>[2x]VFPCSVYVPDEWEVSREKITLLRELGQGSFGMVYEGNARDIIKGEAETRVAVKTVNESASLRERIEFLNEASVMKGFTCH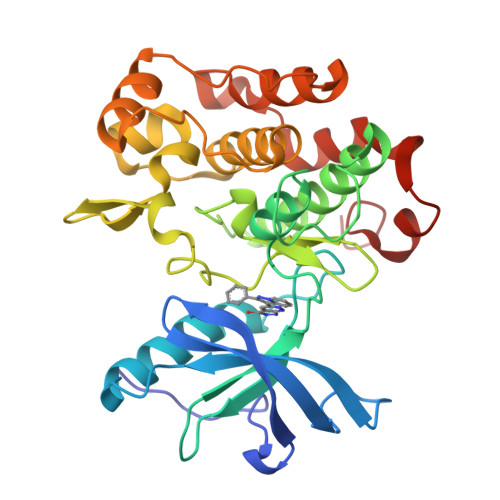HVVRLLGVVSKGQPTLVVMELMAHGDLKSYLRSLRPEAENNPGRPPPTLQEMIQMAAEIADGMAYLNAKKFVHRDLAARNCMVAHDFTVKIGDFGMTRDIYETDYYRKGGKGLLPVRWMAPESLKDGVFTTSSDMWSFGVVLWEITSLAEQPYQGLSNEQVLKFVMDGGYLDQPDNCPERVTDLMRMCWQFNPNMRPTFLEIVNLLKDDLHPSFPEVSFFHSEENK> TQGNTCGGETCSAAQVCLKGKCVCNEVHCRIRCKYG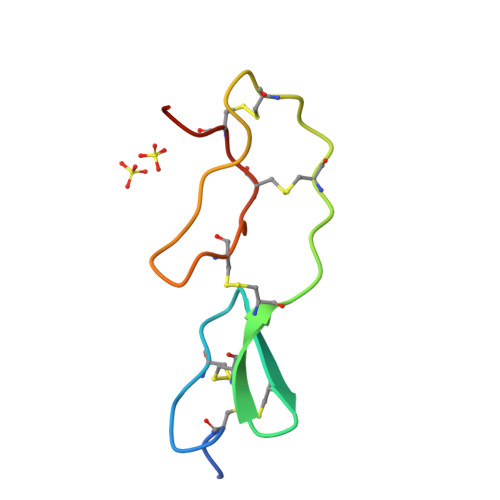LKKDENGCEYPCSCAKASQ>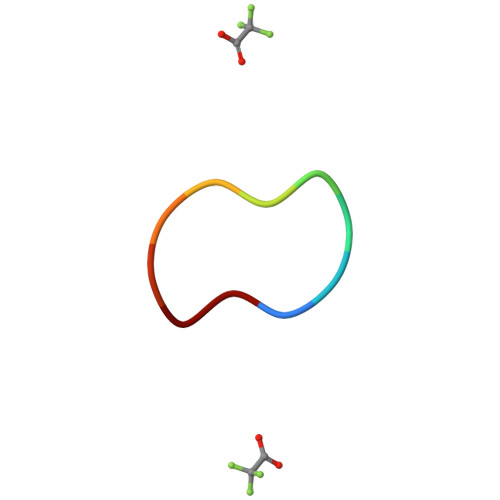 EPPKVEPPKV> RGSHHHHHHGSVKIVTSQAEFDSIISQNELVIVDFFAEWCGPSKRIAPFYEECSKTYTKMVFIKVDVDEVSEV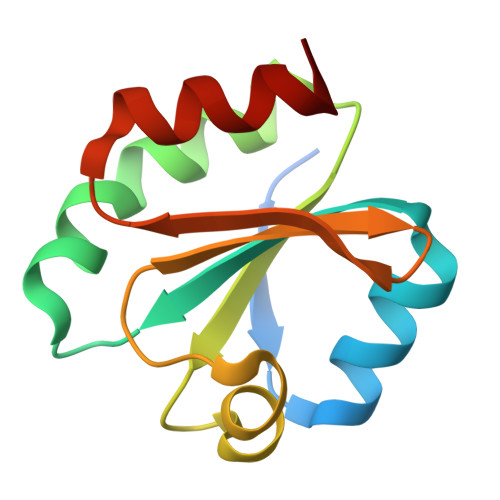TEKENITSMPTFKVYKNGSSVDTLLGANDSALKQLIEKYAA2-ethyl-1,2,3,4-tetrahydroisoquinolin-5-amine 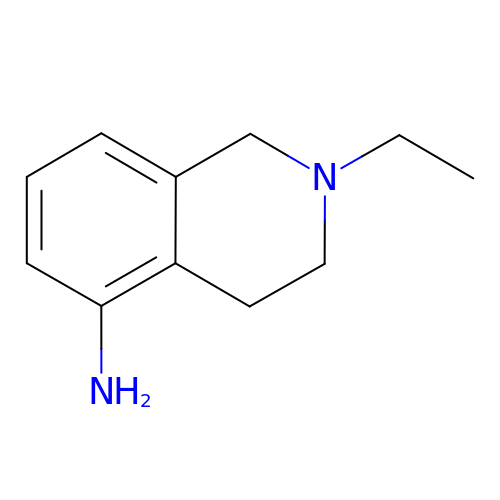| C11 H16 N2 | BQEJAFIVZNAXGW-UHFFFAOYSA-N> SASFAPECTDLKTKYDSCFNEWYSEKFLKGKSVENEC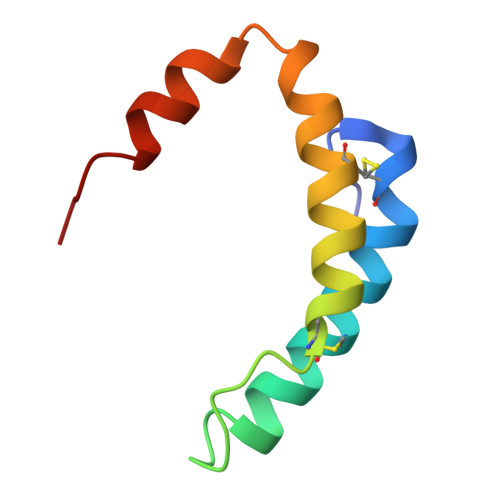SKQWYAYTTCVNAALVKQGIKPALDEAREEAPF>MGSSYHHHHHHSSGENLYFQHMKHGRVFIIKSYSEDDIH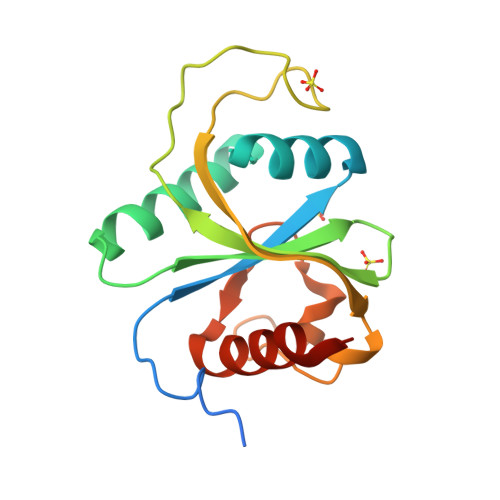RSIKYNIWCSTEHGNKRLDAAYRSMNGKGPVYLLFSVNGSGHFCGVAEMKSAVDYNTCAGVWSQDKWKGRFDVRWIFVKDVPNSQLRHIRLENNENKPVTNSRDTQEVPLEKAKQVLKIIASYKHTTS[2x]3-[({2-[2-(1H-imidazol-1-yl)pyrimidin-4-yl]ethyl}amino)methyl]benzonitrile | C17 H16 N6 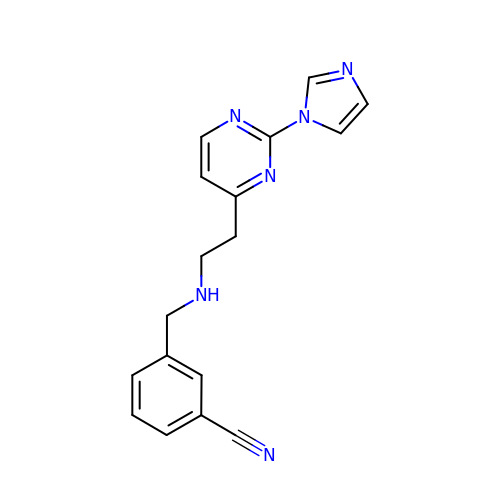| ODSRQJVZWSSZFG-UHFFFAOYSA-N Syntenin-1, a member of the PDZ domain-containing scaffold protein family, is involved in diverse physiological processes, such as cell adhesion, protein trafficking10, and transcription factor activation. Syntenin-1 is an adaptor-like molecule that contains at least four separate structural domains: An N-terminal domain, two tandem PDZ domains (PDZ1 and PDZ2), and a C-terminal region. The diverse biological functions of syntenin-1 arise from its ability to bind the cytoplasmic domains of numerous physiologically relevant signaling and adhesion molecules, including syndecans, neurexins, and ephrin B12131415. The present study provides clear evidence that syntenin-1 negatively regulates syndecan-4 signaling via binding between syndecan-4 and the syntenin-1 PDZ2 domain.

The crystal structures of syntenin-1 with and without a syndecan-4 cytoplasmic domain peptide (corresponding to the C2 region; 4C2) were determined to be 2.8 and 1.9 Å, respectively. Surprisingly, our analysis of the syntenin-1/4C2 complex revealed that syntenin-1 formed a symmetrical pair of dimers, each of which was anchored by a syndecan-4 dimer. Each syndecan-4 bridged two syntenin-1 dimers, forming a unique dimer-of-dimers topology. Our crystal structure analysis of the syntenin-1/4C2 complex showed that a major interaction between syntenin-1 and syndecan-4 originated from hydrophobic forces between syndecan-4 residues, Y201 and A202, and syntenin-1 residues, H210 and V211. Upon syndecan-4 binding, a structural rearrangement of the PDZ2 domain provided a specific binding pocket for the syndecan-4 cytoplasmic domain. PDZ1 helix-2 (α2) also underwent rearrangement upon syndecan-4 binding. Structurally, the C-terminal region of syntenin-1 was found to form a short α-helix (α5), and residues P273, F277, E278, I280, and I281 of α5 were observed to participate in molecular interactions with residues of PDZ1 and PDZ2, thereby stabilizing the syntenin-1/4C2 complex. Notably, the F275 of one α5 interacted with that of the other subunit. Moreover, the C-terminal region of syntenin-1 induced a large conformational change that triggered inter-dimeric interactions between the α2 helices of the PDZ1 domains with a salt bridge between D174 and K178. The crystal structure of the syntenin-1/4C2 complex revealed a bona fide architecture in which the syndecan-4 dimer bridges the dimer-of-dimers of syntenin-1.

>[2x]GSAMADIGAEIKQGIREVILCKDQDGKIGLRLKSVDNGIFVQLVQANSPASLVGLRFGDQVLQINGENCAGWSSDKAHKVLKQAFGEKITMTIRDRPFERTVTMHKDSSGHVGFIFKSGKITSIVKDSSAARNGLLTDHHICEINGQNVIGLKDAQIADILSTAGTVVTITIMPAFIFEHIIKRMAPSIMKSLMDHTIPEV;>[2x]APTNEFYA>[2x]GPHMTDKSDRTDWVALMRAIRDHRDEAAFAELFQHFAPKVKGFLMKSGSVASQAEECAQDVMATVWQKAHLFDPSRASVATWIFTIARNRRIDGLRKDRQPEPEDLFWGPDSEPDQADVYEMQQENARLGRAIARLPEAQRALIERAFFGDLTHRELAAETGLPLGTIKSRIRLALDRLRQHMS;>MTIRH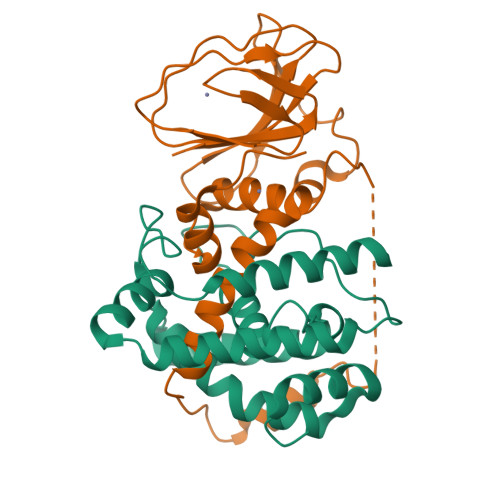HVSDALLTAYAAGTLSEAFSLVVATHLSLCDECRARAGALDAVGGSLMEETAPVALSEGSLASVMAQLDRQIQRPAPARRADPRAPAPLADYVGRRLEDVRWRTLGGGVRQAILPTGGEAIARLLWIPGGQAVPDHGHRGLELTLVLQGAFRDETDRFGAGDIEIADQELEHTPVAERGLDCICLAATDA[2x]>[2x]GSHMTEAEYLANYDPKAFKAQLLTV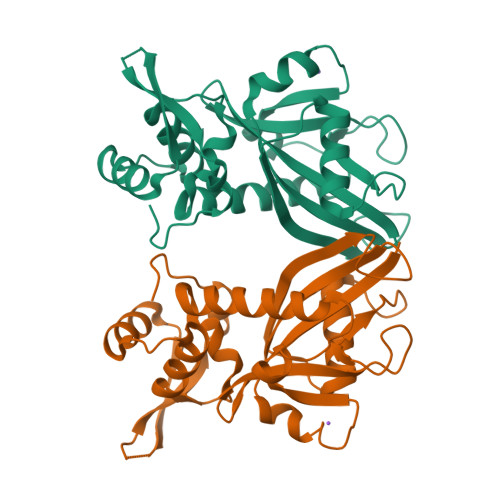DAVLFTYHDQQLKVLLVQRSNHPFLGLWGLPGGFIDETCDESLEQTVLRKLAEKTAVVPPYIEQLCTVGNNSRDARGWSVTVCYTALMSYQACQIQIASVSDVKWWPLADVLQMPLAFDHLQLIEQARERLTQKALYSLVPGFALSEPFTLPELQHVHEVLLGKPIQGKSFRRRVEQADLLIDTGLKRTERGRPANLYCLKPDTASYRFLRNLEC>MSSSYDEASLAPEETTDSFWEVGNYKRTVKRIDDGHRLCNDLMNCVQERAKIEKAYGQQLTDWAKRWRQLIEKGPQYGSLERAWGAIMTEADKVSELHQEVKNNLLNEDLEKVKNWQKDAYHKQIMGGFKETKEAEDGFRKAQKPWAKKMKELEAAKKAYHLACKEEKLAMTREMNSKTEQSVTPEQQKKLQDKVDKCKQDVQKTQEKYEKVLEDVGKTTPQYMENMEQVFEQCQQFEEKRLVFLKEVLLDIKRHLNLAENSSYIHVYRELEQAIRGADAQEDLRWFRSTSGPGMPMNWPQFEEWNP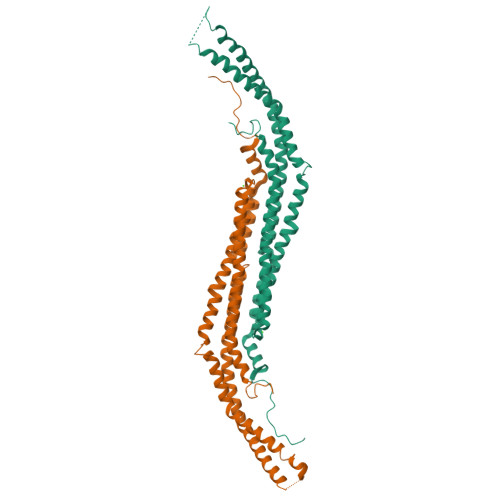[2x]>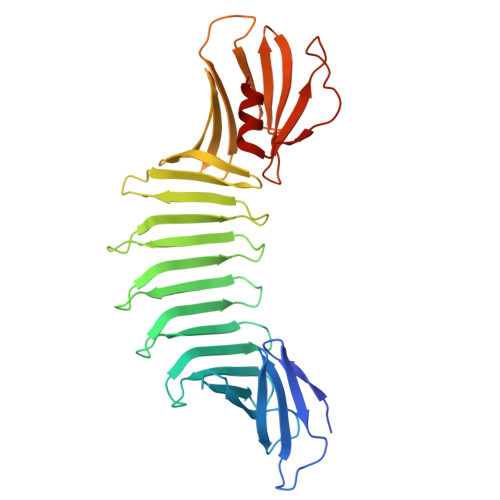 GSHMKNSVSVDLPGEMKVLVSKEKNKDGKYDLIATVDKLELKGTSDKNNGSGVLEGVKADKSKVKLTISDDLGQTTLEVFKEDGKTLVSKKVTSKDKSSTEEKFNEKGELSEKKITRADKSSTEEKFNEKGELSEKKITRADKSSTEEKFNEKGEVSEKIITRADGTRLEYTGIKSDGSGKAKEVLKGYVLEGTLTAEKTTLVVKEGTVTLSKNISKSGEVSVELNDTDSSAATKKTAAWNSGTSTLTITVNSKKTKDLVFTKENTITVQQYDSNGTKLEGSAVEITKLDEIKNALK> MATLTDRTYLPPLEDCLTGRTVILSWRLVASALEDADLARLTSPALSTFLRDGFVHELLKHPARVFEPKDLKQEFETKTSSIQTVAPGVDTIKKDALWLADAVAINQVAALRIVLIEYQTRAHSHLVLPLSTQDVANIQEAAGVGDAHASSILSLLNPASAVDAETMWCDFETEARRRERILATYLSERRSFTAAVDALVTFLLHSAPGQHKDLDSLRRALLKDAFAFDEDLDVPDRSKLLTMAPTYMNLVEDCIARAQALPAKLGESFKTEAFELDWLRTAITEAVHSLSIAFQALDLDTPYFAPHELLSEWFELMNSSLFLESILGFEVVADLAMPARSLVSAICLKMLNIDRTIQFLHDFDYPDGEEPYLLSSQTLNKIHTAVTNAVNSGVA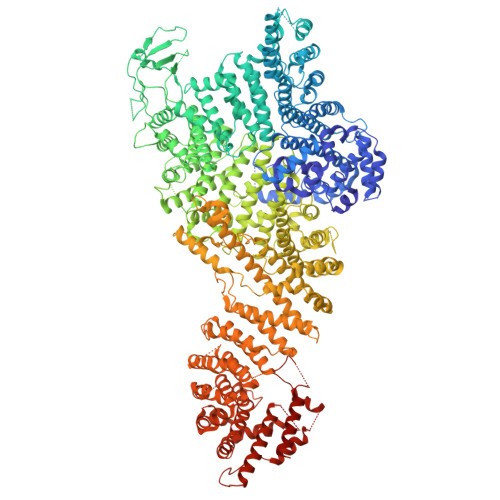ASLPVAFAWSLIVHQMHLGYQERAERRDLLVNQRAQAGFELEFQPSASTPNRRRRNSAGSIVSLEASPYDDFLREQRLDNDIAPVEQIAMLATSRGQVYQVMSEMALCLGTTHEAAFRPAVGARARLVFQDLLKRAAYLIPYQDEPVFSLLAILATGRQYWDVTDALSASSLNQVYTDMLDDETLFTQFTMQAINRFPYEFNPFSVLCRVLAAALITNKDKADVVTGWLWRTPTLTVDWNPAWDRSYELCFEDENTNSFRLTRDVDLFGSASPARPRHLAAEERFIIPEGTLGRFVTDVGRTARLEFEHSALALLGKRLEVKAAEEICDSGMAPLDVDEQAEAVAMLATVLRAESLKSTAKGGDPEAPLKFLKEASRLLPHNKDILTVISDTIDGLVEKELLELDGPQIAVLASCLQFLHAALAVCPGRVWAYMSRCALIAGDARPGRLSRITGSLDMYAERFDLLSSAVKLFAALIDSAACSAVQRRAGSTALVSVRSAVENPWLGTSEKILSRVALAIAQAALDVYESTTTWRFRSELDRSILVRDVVGLMHKLVVHAHTLSSHLTSTLSPAAAHIISSFLTPPPSASSLRFQPLLGTLLVALITPRATLYPGQSRILAERVTSVLAFCTSLLRAADFLGQTHIPLQTHLFQSACLLARLPAANAVYRAPVLELLRALVEVAGRAANGSGEPPSLLGYLGSHAARSFISLVEGIDKPFGRVEHAVVTWRFFAAVIRNRQQWMAGCLLTGRTPREALKGGGEQKIERKVGEGSVLAAAMERLREVKSLDVQEAVAVMDFVVSAQNYWPWTIFAVRKEKEVVDALRGYVRGLKAPGMVMKTDGAAAAAFQARIAAYVAETFAMQLYHMRQMRQAEKFAGELVADLDYFLREGVMVWGYNASLHGNFARNFAKRFPGVEVDDFKRTMWLPRELGKGYYYALEVAEQMLGFDAGWGGVKQSGFRKEMETANLNLSLVEAQVSLFHAWEYLLLELTLSLLPKKENAAFARQVLQVVEQCLEANQRSQPPENIFVVLGHARAGLALTLLQRLADANQLPRDVTHLLALVSSAIHAVENPFGANDLPYFRTLLKILFVVLRAAKQGTAKPGESNVAITQQVLTILDRVVARCFRALAALVHEQQQNATDGTTTAPEDLALITAILQACLSVPGIEQCQVQVLNIMAAHDVFQVAVALFSWADRLLPANPSPASSSTSTSATNPASGDPVYGELALLFLLELSALPALAEHLACDGLLGHLAAARLAGYMRRTNVGPFAENAGAARCYAIWAKCLLPLLLNILAALGSTVAPEVAWVLNQFPNLLQSSVERIEPPGFSRPTLSLASTPPRQKFISLLEISEIHSLALLTRVLAACRAQNARDVPEVTWDGAKVLECVEYWLRGRKVLRERLVPLGPREVEWRGMVATGGVVGVAGDGGEGCENRLEEKAVGLLVGVREVLEGGLEGEGE By administering enzyme drugs called L-asparaginases, which act to quickly deplete Asn in the blood, this drug specifically impacts ALL cells, starving them to death while leaving normal cells largely intact. WoA, like most bacterial Type II L-asparaginases, is a tetramer built by a dimer-of-dimer with 330 residues per protomer. In our structures we observe that the overall fold of each protomer follows the general two-domain fold of bacterial type II L-asparaginases. We sought to clarify this question and to further explain the substrate discrimination, if there is any, between the two forms, by solving the crystal structures of both variants in complex with either the product Asp or L-glutamic acid (Glu).

Surprisingly, we observed unambiguous electron density for an open conformation of the flexible loop in the other three structures, WoA-P121 + Glu, WoA-S121 + Asp and WoA-S121 + Glu. Likewise, both WoA variants soaked in a Glu solution had ligand bound but the open loop conformation. Overlay of WoA-P121 + Glu and WoA-S121 + Glu showed identical Glu binding mode. In this comparison, WoA-P121 + Asp represents the closed/active state of the enzyme (pink), whereas WoA-P121 + Glu represents the open/inactive state (green). As the catalytically-relevant state is the one where the N-terminal loop is closed, to better understand how WoA-P121 would accommodate Glu in its closed state, we modelled into the open WoA-P121 + Glu structure the closed loop conformation as observed in the WoA-P121 + Asp structure. This modelling reveals that whereas Asp fits without strain into the closed active site, binding of the larger ligand Glu (Glu has an extra methylene group relative to Asp) seems to be incompatible with loop closure due to several steric clashes. First, whilst the Asp Cβ atom adopts a conformation keeping it in a compatible distance (3.7 Å) from Tyr27, the Glu Cβ atom adopts the opposite conformation that would bring it a relatively short distance of ~3 Å to Tyr27. Second, the active conformation taken by Thr14 in the WoA-P121 + Asp closed structure is not compatible with neither the Cβ, Cγ nor Cδ atoms of Glu (modelled distances of ~1.4 to 1.9 Å). In such an analysis, our theoretical model shows that upon loop closure favourable interactions between Pro121 and Tyr27 would be made. In contrast, the L-glutaminase rates at either saturated substrate concentration or at 0.5 mM – the physiological blood concentration of Gln – were ~8 fold higher in WoA-P121 compared to WoA-S121.

>MAKPQVTILATGGTIAGSGESSVKSSYSAGAVTVDKLLAAVPAINDLATIKGEQISSIGSQEMTGKVWLKLAKRVNELLAQKETEAVIITHGTDTMEETAFFLNLTVKSQKPVVLVGAMRPGSSMSADGPMNLYNAVNVAINKASTNKGVVIVMNDEIHAAREATKLNTTAVNAFASPNTGKIGTVYYGKVEYFTQSVRPHTLASEFDISKIEELPRVDILYAHPDDTDVLVNAALQAGAKGIIHAGMGNGNPFPLTQNALEKAAKSGVVVARSSRVGSGSTTQEAEVDDKKLGFVATESLNPQKARVLLMLALTKTSDREAIQKIFSTY[4x]> 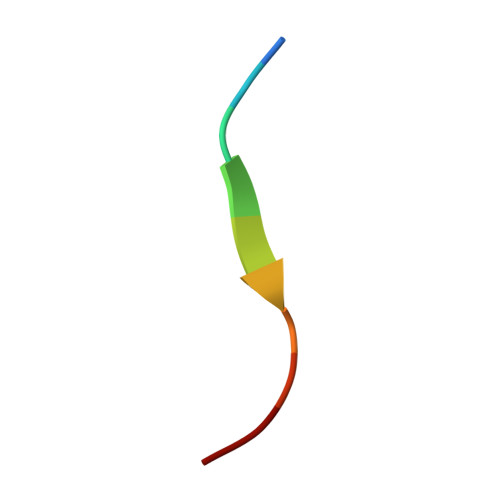TENLYFQSGT> GPMASQPNSSAKKKEEKGKNIQVVVRCRPFNLAERKASAHSIVECDPVRKEVSVRTGGLADKSSRKTYTFDMVFGASTKQIDVYRSVVCPILDEVIMGYNCTIFAYGQTGTGKTFTMEGERSPNEEYTWEEDPLAGIIPRTLHQIFEKLTDNGTEFSVKVSLLEIYNEELFDLLNPSSDVSERLQMFDDPRNKRGVIIKGLEEITVHNKDEVYQILEKGAAKRTTAATLMNAYSSRSHSVFSVTIHMKETTIDGEELVKIGKLNLVDLAGSENIGRSGAVDKRAREA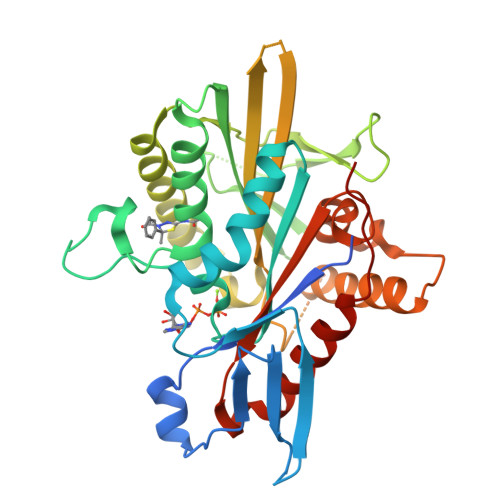GNINQSLLTLGRVITALVERTPHVPYRESKLTRILQDSLGGRTRTSIIATISPASLNLEETLSTLEYAHRAKNILNKPEVNQK>SNASADAQSFLNRVCGVSAARLTPCGTGTSTDVVYRAFDIYNDKVAGFAKFLKTNCCRFQEKDEDDNLIDSYFVVKRHTFSNYQHEETIYNLLKDCPAVAKHDFFKFRIDGDMVPHISRQRLTKYTMADLVYALRHFDEGNCDTLKEILVTYNCCDDDYFNKKDWYDFVENPDILRVYANLGERVRQALLKTVQFCDAMRNAGIVGVLTLDNQDLNGNWYDFGDFIQTTPGSGVPVVDSYYSLLMPILTLTRALTAESHVDTDLTKPYIKWDLLKYDFTEERLKLFDRYFKYWDQTYHPNCVNCLDDRCILHCANFNVLFSTVFPPTSFGPLVRKIFVDGVPFVVSTGYHFRELGVVHNQDVNLHSSRLSFKELLVYAADPAMHAASGNLLLDKRTTCFSVAALTNNVAFQTVKPGNFNKDFYDFAVSKGFFKEGSSVELKHFFFAQDGNAAISDYDYYRYNLPTMCDIRQLLFVVEVVDKYFDCYDGGCINANQVIVNNLDKSAGFPFNKWGKARLYYDSMSYEDQDALFAYTKRNVIPTITQMNLKYAISAKNRARTVAGVSICSTMTNRQFHQKLLKSIAATRGATVVIGTSKFYGGWHNMLKTVYSDVENPHLMGWDYPKCDRAMPNMLRIMASLVLARKHTTCCSLSHRFYRLANECAQVLSEMVMCGGSLYVKPGGTSSGDATTAYANSVFNICQAVTANVNALLSTDGNKIADKYVRNLQHRLYECLYRNRDVDTDFVNEFYAYLRKHFSMMILSDDAVVCFNSTYASQGLV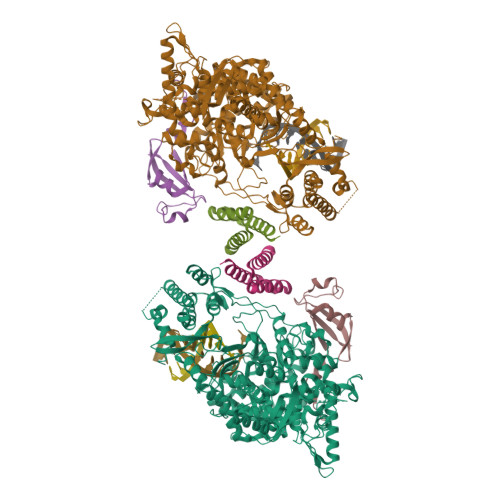ASIKNFKSVLYYQNNVFMSEAKCWTETDLTKGPHEFCSQHTMLVKQGDDYVYLPYPDPSRILGAGCFVDDIVKTDGTLMIERFVSLAIDAYPLTKHPNQEYADVFHLYLQYIRKLHDELTGHMLDMYSVMLTNDNTSRYWEPEFYEAMYTPHTVLQ[2x];>[2x]SNAAIASEFSSLPSYAAFATAQEAYEQAVANGDSEVVLKKLKKSLNVAKSEFDRDAAMQRKLEKMADQAMTQMYKQARSEDKRAKVTSAMQTMLFTMLRKLDNDALNNIINNARDGCVPLNIIPLTTAAKLMVVIPDYNTYKNTCDGTTFTYASALWEIQQVVDADSKIVQLSEISMDNSPNLAWPLIVTALRANSAVKLQ;>[2x]SNASKMSDVKCTSVVLLSVLQQLRVESSSKLWAQCVQLHNDILLAKDTTEAFEKMVSLLSVLLSMQGAVDINKLCEEMLDNRATLQ> LWMHKVPAS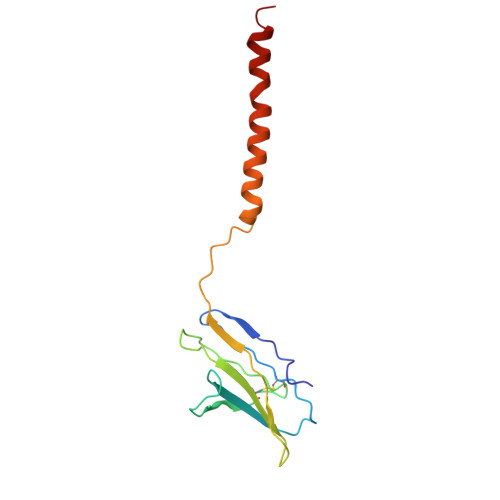LMVSLGEDAHFQCPHNSSNNANVTWWRVLHGNYTWPPEFLGPGEDPNGTLIIQNVNKSHGGIYVCRVQEGNESYQQSCGTYLRVRQPPPRPFLDMGEGTKNRIITAEGIILLFCAVVPGTLLLFRKRW>MAGVPFRSPSTGRNVRAVLFDTFGTVVDWRTGIATAVADYAARHQLEVDAVAFADRWRARYQPSMDAILSGAREFVTLDILHRENLDFVLRESGIDPTNHDSGELDELARAWHVLTPWPDSVPGLTAIKAEYIIGPLSNGNTSLLLDMAKNAGIPWDVIIGSDINRKY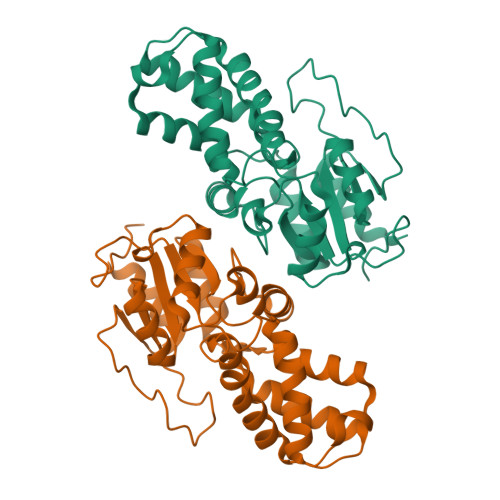KPDPQAYLRTAQVLGLHPGEVMLAAAHNGDLEAAHATGLATAFILRPVEHGPHQTDDLAPTGSWDISATDITDLAAQLRAGSTGFR[8x]>MSQTSLTPGQRFREAVATEHPLQVVGTINANHALLAKRAGFKAIYLSGGGVAAGSLGLPDLGISGLDDVLTDVRRITDVCDLPLLVDVDTGFGSSAFNVARTVKSMIKFGAAAMHIEDQVGAKRCGHRPNKEIVSQQEMVDRIKAAVDARSDDSFVIMARTDALAVEGLQAAIDRACACVEAGADMIFPEAMTELAMYKEFAAAVKVPVLANITEFGATPLFTTDELASADVSLVLYPLSAFRAMNKAAENVYTAI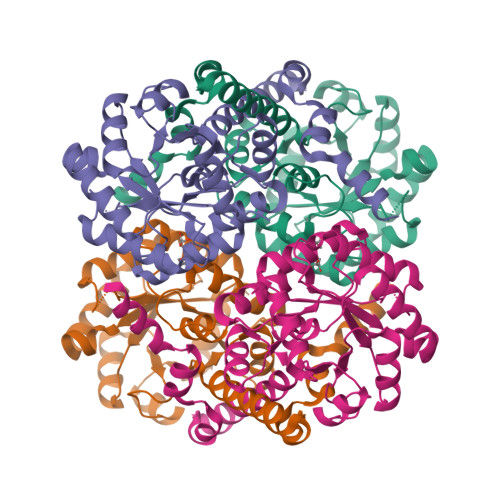RRDGTQKNVIDTMQTRMELYDRIDYHSFEQKLDALFAQKKNA[4x]L-tagatose | C6 H12 O6 | 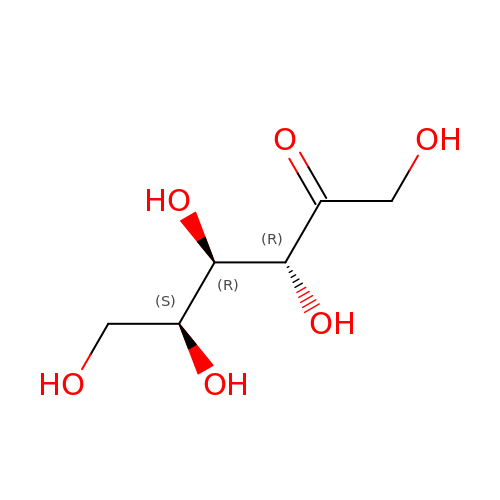BJHIKXHVCXFQLS-LFRDXLMFSA-N>[2x]GSMALTQVETEIVPVSVDGETLTVEAVRRVAEERATVDVPAESIAKAQKSREIFEGIAEQNIPIYGVTTGYGEMIYMQVDKSKEVELQTNLVRSHSAGVGPLFAEDEARAIVAARLNTLAKGHSAVRPIILERLAQYLNEGITPAIPEIGSLGA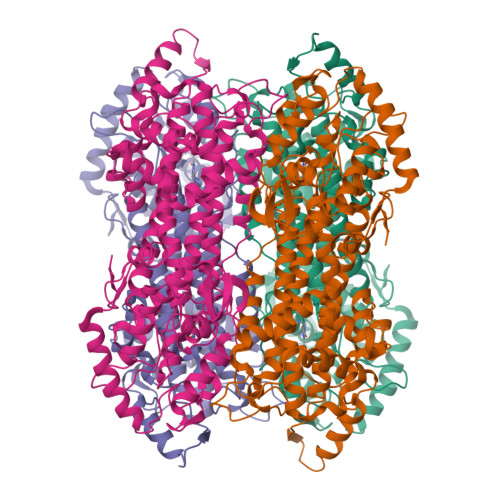SGDLAPLSHVASTLIGEGYVLRDGRPVETAQVLAERGIEPLELRFKEGLALINGTSGMTGLGSLVVGRALEQAQQAEIVTALLIEAVRGSTSPFLAEGHDIARPHEGQIDTAANMRALMRGSGLTVEHADLRRELQKDKEAGKDVQRSEIYLQKAYSLRAIPQVVGAVRDTLYHARHKLRIELNSANDNPLFFEGKEIFHGANFHGQPIAFAMDFVTIALTQLGVLAERQINRVLNRHLSYGLPEFLVSGDPGLHSGFAGAQYPATALVAENRTIGPASTQSVPSNGDNQDVVSMGLISARNARRVLSNNNKILAVEYLAAAQAVDISGRFDGLSPAAKATYEAVRRLVPTLGVDRYMADDIELVADALSRGEFLRAIARETDIQLR> MSRNYVVAGYVSDRHLPELTKEELKKLTHINIAFGHVREDRIQTGHLQNLKLLPELKRENPDLTILLSVGGWSAGGFSEAASTEAG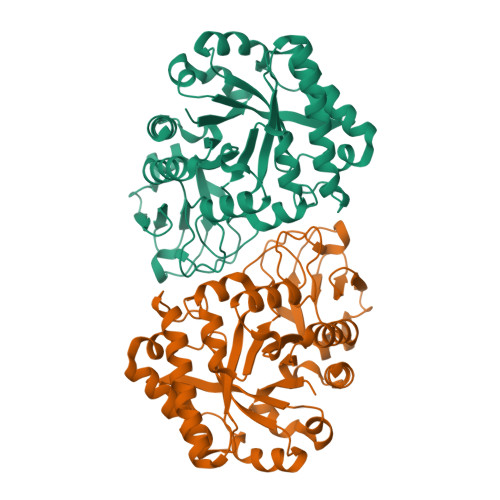RQAMAESAVRAVTEYALDGVDLDWEYPCYAEAGIAASPDDKANFTLLLRTMREALDRQGERDGRHYWLTIAAGADQYYIDGTEMAEVQRYLDFVQLMTYDMRGGFQTLTGHHTNLYTGTGDLFRISVDASVNLFVRAGVPKEKIVIGAAFYSRMWKDVPNVNRGLYQMSPGSGGYGPDFTELAAEYIDRNGFVRYWDEEAKAPYLFDGQTFISYDDEMSIRYKCDYVKAQELAGVMFWEYGCDRTHRLLDALYQGLQSS> GELVRTDSPNFLCSVLPTHWRCNKTLPIAFKVVAKGDVPDGTLVTVMAGNDENYSAELRNATAAMKNQVARFNDLRFVGRSGRGKSFTLTITVFTNPPQVATYHRAIKITGDGPR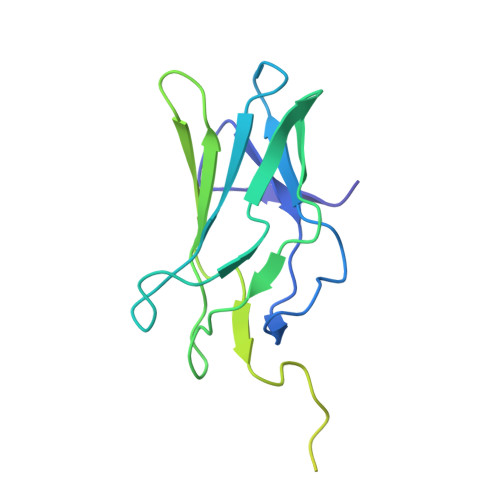EPRRHRQKLDDQTKPGSLSFSERLSELEQLRRTAMRVSPHHPAPTPNPRASLNHSTAFNPQPQSQMQDARQIQPSPPWSYDQSYQYLGS>[8x]MSCKPNILVLFYGYGSIVELAKEIGKGAEEAGAEVKIRRVRETLPPEFQSRIPFDKVKDIPEVTLDDMRWADGFAIGSPTRYGNMAGGLKTFLDTTAILWKDNVLYG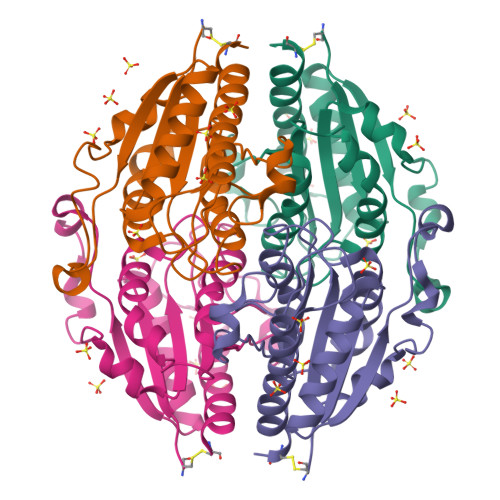KPVTFFTEASTVHGGHETTILTMSTYAYHFGMIIVPIGYGIPELFQTTTGGGPYGATHLGSKEELDEMERKIARFQGKRITEVAKAIKCCNK>GSDRPTPVPLPNSEQF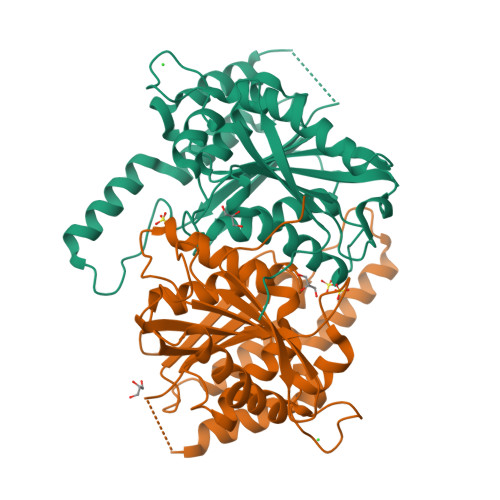YLENDRGEPYLIQVSWPLHWEDKQTGRGPLPIIYIVDGNALFLTATEAAWRRAAASHFAGGGIIVAIGYPLKGKLYDARRRSFDLTPPTACAPVGYGGADVFLDFIENSVRPAVQARFPQVSLAREALYGHSYGGLLALHALFTRPQSFDCYIASSPSIWWNSLCILHEAKAFVETKKVSHDQSPSLMVSWGSWQQHPPRWADELLDHYEARKRTAAELRMADNALDLCAMLHGCSRLHALIKTEYEGEDHTSVMSCSVSRGLTMFFEDWPFHQSG[2x]>[3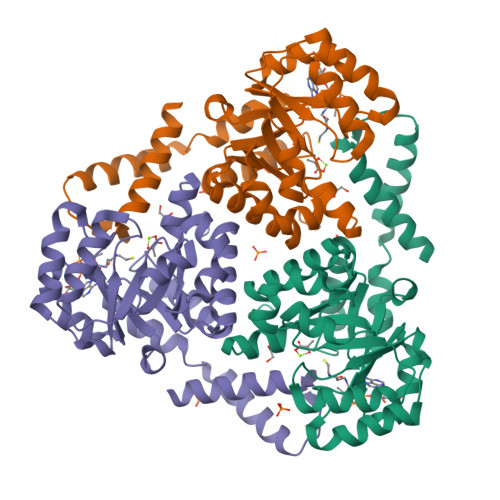x]MAHHHHHHMNLRAAGPGWLFCPADRPERFAKAAAAADVVILDLEDGVAEAQKPAARNALRDTPLDPERTVVRINAGGTADQARDLEALAGTAYTTVMLPKAESAAQVIELAPRDVIALVETARGAVCAAEIAAADPTVGMMWGAEDLIATLGGSSSRRADGAYRDVARHVRSTILLAASAFGRLALDAVHLDILDVEGLQEEARDAAAVGFDVTVCIHPSQIPVVRKAYRPSHEKLAWARRVLAASRSERGAFAFEGQMVDSPVLTHAETMLRRAGEATSE>AAASMSALITENMHMKLYMEGTVNNHHFKCTSEGEGKPYEGTQTMRIKVVEGGPLPFAFDILATSFMYGSKTFINHTQGIPDFFKQSFPEGFTWERVTTYEDGGVLTATQDTSLQDGCLIYNVKIRGVNFPS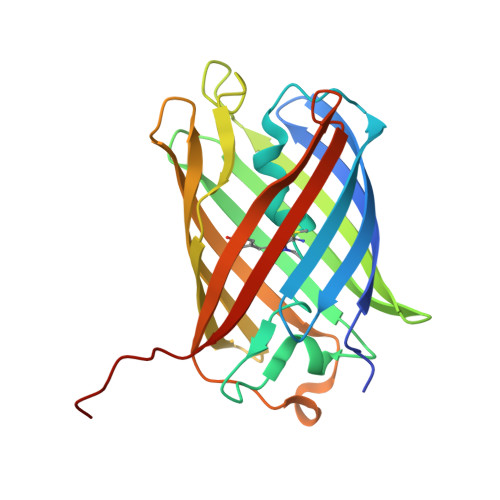NGPVMQKKTLGWEACTEMLYPADGGLEGRADMALKLVGGGHLICNLKTTYRSKKPAKNLKMPGVYYVDRRLERIKEADKETYVEQHEVAVARYCDLPSKLAHK[4x]>HMYRNVPIWAQKWKPTIKALQSINVKDLKIDPSFLNIIPDDDLTKSVQDWVYATIYSIAPELRSFIELEMKFGVIIDAKGPDRVNPPVSSQCVFTELDAHLTPNIDASLFKELSKYIRGISEVTENTGKFSIIESQTRDSVYRVGLSTQRPRFLRMSTDIKTGRVGQFIEKRHVAQLLLYSPKDSYDVKISLNLELPVPDNDPPEKYKSQSPISERTKDRVSYIHNDSCTRIDITKVENHNQNSKSRQSETTHEVELEINTPALLNAFDNITNDSKEYASLIRTFLNNGTIIRRKLSSLSYEIFEGSKKV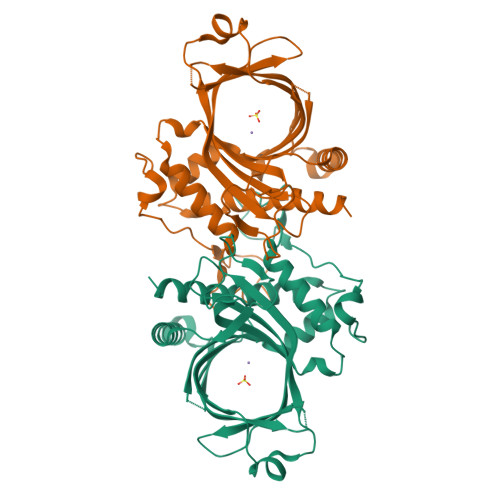M[3x]> MANPYERGPDPTESSIEAVRGPFAVAQTTVSRLQADGFGGGTIYYPTDTSQGTFGAVAISPGFTAGQESIAWLGPRIASQGFVVITIDTITRLDQPDSRGRQLQAALDHLRTNSVVRNRIDPNRMAVMGHSMGGGGALSAAANNTSLEAAIPLQGWHTRKNWSSVRTPTLVVGAELDTIAPVSSHSEAFYNSLPSDLDKAYMELRGASHTVSNTPDTTTAKYSIAWLKRFVDKDLRYEQFLCPAPDDFAISEYRSTCPFHHHHHH

Plastic pollution has become a global environmental challenge, driving interest in enzymatic polyethylene terephthalate (PET) recycling by using polyester hydrolases. Metagenome-derived polyester hydrolases, such as LCC and PHL7, have garnered significant attention due to their high activity at elevated temperatures of up to 70 °C. Their engineering led to the development of optimized variants, including LCCICCG, LCC-A2, Turbo-PETase, and PHL7mut3. , PHL7mut3 has been designed to improve the activity and thermostability of PHL7 by the Q175E, L210T, and D233 K mutations. In this study, the PHL7 wild-type enzyme and the improved PHL7 triple mutant PHL7mut3 were expressed in E. coli and P. pastoris, and their PET-degrading activity under various conditions as well as their thermal stability was assessed. Both the PHL7 and the PHL7mut3 sequences contain three putative N-glycosylation sites (N143, N144, and N161). To assess the impact of mutations and glycosylation on structural folding, we used X-ray crystallography to determine the structures of PHL7mut3, expressed in both E. coli (E_PHL7mut3) and P. pastoris (P_PHL7mut3), as well as a non-glycosylated variant with three additional mutations (P_PHL7mut3_ng), also expressed in P. pastoris.

For P_PHL7mut3, the glycosylation of N143 was observed. Two N-acetyl-glucosamine residues could be modeled, but not the additional residues of the glycan chain, likely due to disorder. N143 adopted two distinct conformations, with glycan attachment observed only in conformation A. The occupancy was refined to 0.72 for the first N-acetyl glucosamine unit and 0.56 for the second. The electron density for residues N161 and N144 showed no evidence of glycosylation. N144 is more buried than N143 and it forms hydrogen bridges to Q104 and S146 with its Nδ2 and Oδ1 atoms, respectively. The buried position of N144 might prevent its glycosylation. N161 is involved in crystal contact with residue H264, the penultimate histidine residue of the His-tag of this construct. It is thus conceivable that a fraction of the protein in the crystallization mixture was glycosylated at N161, but only the N161-unglycosylated fraction was enriched in the crystal because glycosylated N161 is not compatible with this crystal form. The N143 glycosylation site is approximately 17 Å away from the substrate binding site, but it is part of the loop that links an α-helix and a β-strand forming part of the active site structure. Thus, glycosylation at N143 might influence the dynamics of the active site.5-fluoro-N-[(2-methyl-1,3-thiazol-5-yl)methyl]pyridin-3-amine | 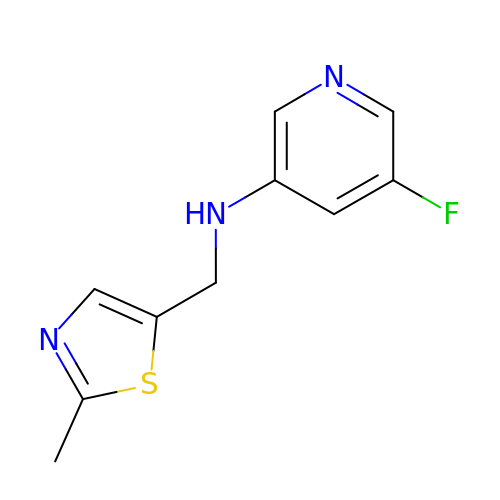C10 H10 F N3 S | SSOIKBIBPGCZFT-UHFFFAOYSA-N>[22x]MAQVINTNSLSLMTQNNLNTSQSALNTAIQRLSSGLRINSAKDDAAGQAIANRFTANIKGLTQAQRNANDGISLAQTTEGALTEVNNNLQRIRELSVQAATGSNSASDLQSIQDEIKQRLEEINRVSEQTQFNGVKVLAKDTKMNIQVGANDGEIIAIDLKEITAKTLGLDGFNVSGPKGTPAALVAADYQAAYGTTTNVTTTAVTESSA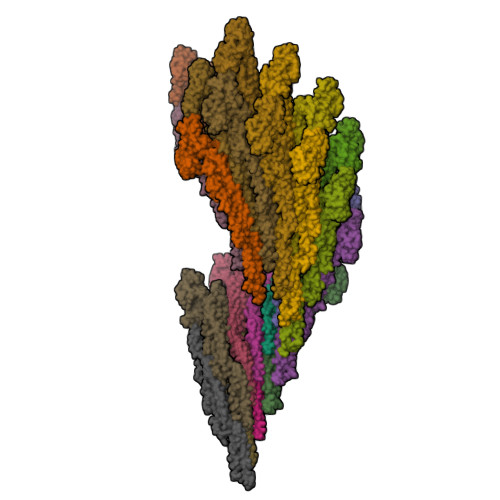NALAGRLGVANGSVALAATAEKDDNGNWYATVTITAGSATEVSTLKAKGFEVENGVAKEFYIALDPQSADVTTTAGTAAFALDTANIQLSSITSGASSNPLAKLDAALADVDTLRSSLGAVQNRFDSVISNLGTTVTNLSASRSRIQDADYATEVSNMTRAQILQQAGTSVLAQANQTTQNVLSLLR>MLILKGTKTVDLSKDELTEIIGQFDRVHIDLGTGDGRNIYKLAINDQNTFYIGIDPVKENLFDISKKIIKKPSKGGLSNVVFVIAAAESLPFELKNIADSISILFPWGTLLEYVIKPNRDILSNVADLAKKEAHFEFVTTYSDSYEEAEIKKRGLPLLSKAY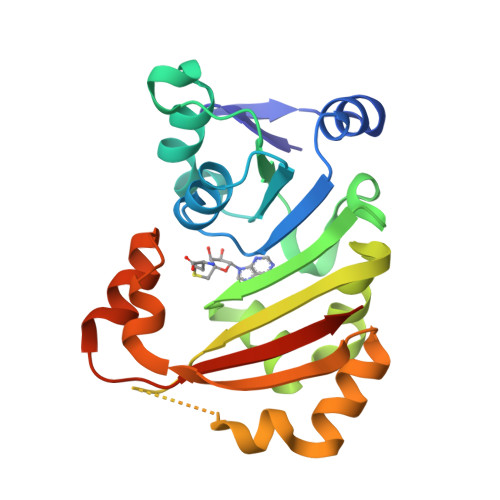FLSEQYKAELSNSGFRIDDVKELDNEYVKQFNSLWAKRLAFGRKRSFFRVSGHVSKHHHHHHH[2x]> SDRVRSITLGNSTITTQECANVVVGYGRWPTYLRDDEATAEDQPTQPDVATCRFYTLDSIKWEKGSVGWWWKFPEALSDMGLFGQNMQYHYLGRAGYTIHVQCNASKFHQGCLLV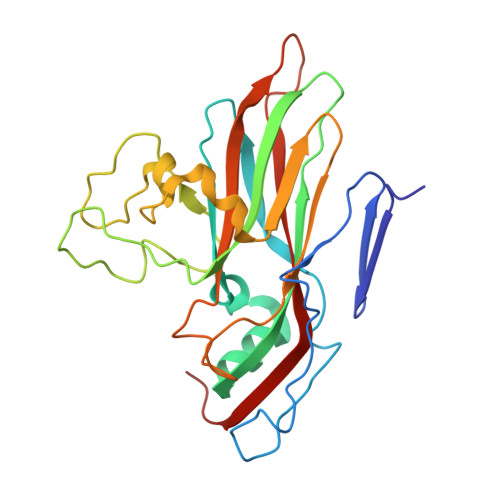VCVPEAEMGGAVVGQAFSATAMANGDKAYEFTSATQSDQTKVQTAIHNAGMGVGVGNLTIYPHQWINLRTNNSATIVMPYINSVPMDNMFRHYNFTLMVIPFVKLDYADTASTYVPITVTVAPMCAEYNGLRLAQ5-acetamido-9-(benzoylamino)-3,5,9-trideoxy-3-fluoro-D-erythro-alpha-L-manno-non-2-ulopyranosonic acid | C18 H23 F N2 O9 | 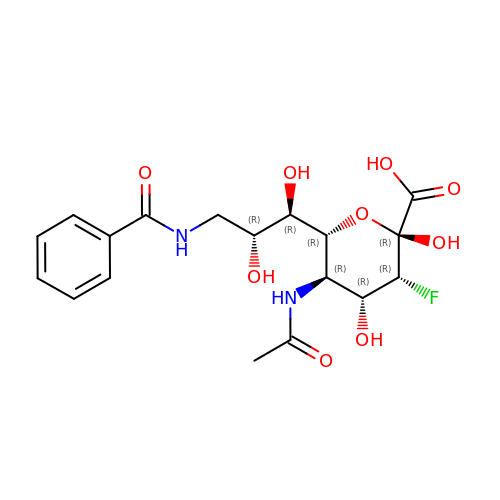MROQLLHLBMWCPR-LQUZZVICSA-N Heat-shock protein 90 (Hsp90) is a highly conserved ATP-dependent molecular chaperone. Hsp90 is a V-shaped homodimer, with each protomer consisting of three major domains: a C-terminal dimerization domain (CTD); a middle domain (MD), which has been linked to client binding; and an N-terminal ATPase domain (NTD). Most higher eukaryotic cells possess four Hsp90 homologs: two cytosolic isoforms, one of which is constitutively expressed while the other is induced by heat shock and stress (Hsp90β and Hsp90α, respectively), one localized to the endoplasmic reticulum (Grp94) and one localized to the mitochondria (TRAP1). Using TRAP1 as a model system for Hsp90, here we investigate how ATP hydrolysis is coupled to its conformational asymmetry and propose a model connecting it to client remodeling.

To generate an ADP-state in only one protomer, we make use of the observation that the MD-Arg (R402 in hTRAP1), the only residue in Hsp90 that contacts the γ-phosphate, acts as an ATP sensor and mutating this residue would effectively mimic the ADP state. To address this concern, we crystallized an equivalent heterodimeric construct of zTRAP1 (+/R417A in zebrafish sequence numbering) in the presence of ADP-BeF. Heterodimeric (+/R417A) zTRAP1 was incubated with 10 mM ADP-BeF/MgCl2 for 1 hr at 30˚C to allow dimer closure. As predicted from the DEER results, the heterodimer adopts an essentially identical asymmetric closed state, and the C-terminal-fused SpyCatcher-SpyTag complex packs against its symmetry mate in the opposing dimer. The structure shows that the R417A mutation does not perturb the overall closed state. To avoid model bias, the dataset was refined starting with alanines replacing arginines at positions 417 on both protomers. The Fo-Fc difference map (insets) show strong positive density for the arginine only on the buckled protomer (ATP state), while the R417A mutation is on the straight protomer (ADP state). This is completely consistent with the interprobe distances measured in the DEER experiments correctly representing the buckled and straight protomer conformations. Altogether, this demonstrates that the loss of the γ-phosphate contact within the closed dimer is a strong determinant of the corresponding protomer conformation. The construct used for heterodimeric zebrafish TRAP1 crystallography (+/R417A) has modified linker lengths appended to its C-terminus to account for the offset in starting amino acid residues between SpyCatcher and SpyTag.

> GIDPFTSTQQHTEPAEEETLHNIITDTENVQGSFSKHEFQAETKKLLDIVARSLYSEKEVFIRELISNGSDALEKLRHRMITAGGDTAPMEIHLQTDSVKGTFTIQDTGVGMNKEDLVSNLGTIARSGSKAFLDALQNQAEASSSIIGQFGVGFYSAFMVADKVEVYSQSAEADAPGYKWSSDGSGVFEVAEASGVRQGTKIVLHLKDDCKEFSSEDRVKEVVTKYSNFVSFPIFLNGRRLNTLQALWMMEPKDISEWQHEEFYRYVAQAYDKPRYTLHYRADAPLNIRSIFYVPEMKPSMFDVSREMGSSVALYSRKILIQTKATDILPKWLRFLRGVVDSEDIPLNLSRELLQESALIRKLRDVLQQRVIRFLLDQSKKDPEKYARFFEDYGLFMREGIVTTGEQSVKEDIAKLLRFESSALPAGQQTSLMEYSSRMKAGTRNIYYLCAPNRHLAEHSPYFEAMKQKDMEVLFCFEQFDELTLLHLREFDRKKLISAETDIVVDHYKEEKFQDSKPASERLSSEQAEDLLAWMRNALVQRVTNIKVTPRLDTHPAMITVLEMGAARHFLRTQQLARSSEERAQILQPTLEINTGHDLIKKLHALKDSNPELAQLLLEQIYDNAMIAAGLNEDPRPMISRLNQLLTRALEKHGSDSATHIKFSKRDEDGKELAGATMELRDSSGKTISTWISDGQVKDFYLYPGKYTFVETAAPDGYEVATAITFTVNEQGQVTVNG;> GIDPFTSTQQHTEPAEEETLHNIITDTENVQGSFSKHEFQAETKKLLDIVARSLYSEKEVFIRELISNGSDALEKLRHRMITAGGDTAPMEIHLQTDSVKGTFTIQDTGVGMNKEDLVSNLGTIARSGSKAFLDALQNQAEASSSIIGQFGVGFYSAFMVADKVEVYSQSAEADAPGYKWSSDGSGVFEVAEASGVRQGTKIVLHLKDDCKEFSSEDRVKEVVTKYSNFVSFPIFLNGRRLNTLQALWMMEPKDISEWQHEEFYRYVAQAYDKPRYTLHYRADAPLNIRSIFYVPEMKPSMFDVSREMGSSVALYSRKILIQTKATDILPKWLRFLRGVVDSEDIPLNLSAELLQESALIRKLRDVLQQRVIRFLLDQSKKDPEKYARFFEDYGLFMREGIVTTGEQSVKEDIAKLLRFESSALPAGQQTSLMEYSSRMKAGTRNIYYLCAPNRHLAEHSPYFEAMKQKDMEVLFCFEQFDELTLLHLREFDRKKLISAETDIVVDHYKEEKFQDSKPASERLSSEQAEDLLAWMRNALVQRVTNIKVTPRLDTHPAMITVLEMGAARHFLRTQQLARSSEERAQILQPTLEINTGHDLIKKLHALKDSNPELAQLLLEQIYDNAMIAAGLNEDPRPMISRLNQLLTRALEKHGGSGSSAHIVMVDAYKPTK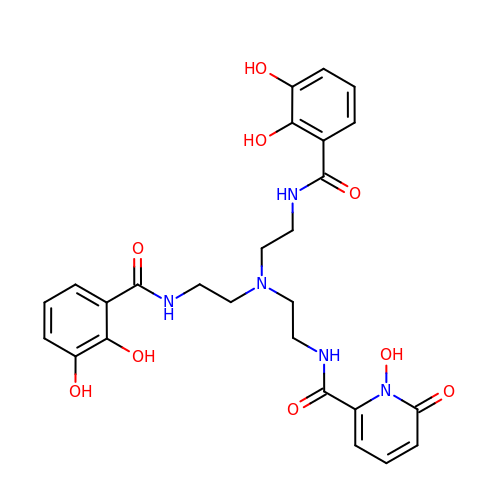N-{2-[bis(2-{[(2,3-dihydroxyphenyl)carbonyl]amino}ethyl)amino]ethyl}-1-hydroxy-6-oxo-1,6-dihydropyridine-2-carboxamide | C26 H29 N5 O9 | SHTLBAYLLAIJDF-UHFFFAOYSA-N> ETFSGGCLFDEPYSTCGYSQSEGDDFNWEQVNTLTKPTSDPWMPSGSFMLVNASGRPEGQRAHLLLPQLKENDTHCIDFHYFVSSKSNSPPGLLNVYVKVNNGPLGNPIWNISGDPTRTWNRAELAISTFWPNFYQVIFEVITSGHQGYLAIDEVKVLGHPCTRTPHFLRIQNVEVNAGQFATFQCSAIGRTVAGDRLWLQGIDVRDAPLKE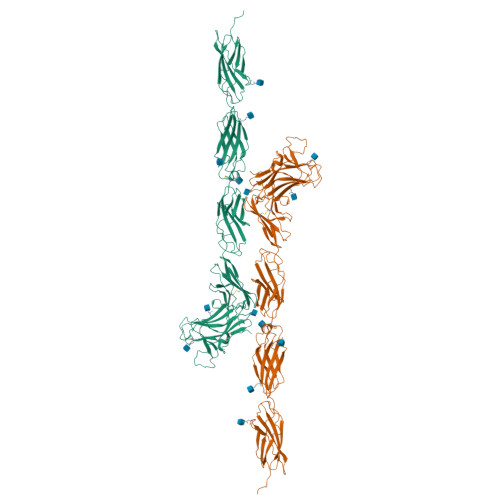IKVTSSRRFIASFNVVNTTKRDAGKYRCMIRTEGGVGISNYAELVVKEPPVPIAPPQLASVGATYLWIQLNANSINGDGPIVAREVEYCTASGSWNDRQPVDSTSYKIGHLDPDTEYEISVLLTRPGEGGTGSPGPALRTRTKCADPMRGPRKLEVVEVKSRQITIRWEPFGYNVTRCHSYNLTVHYCYQVGGQEQVREEVSWDTENSHPQHTITNLSPYTNVSVKLILMNPEGRKESQELIVQTDEDLPGAVPTESIQGSTFEEKIFLQWREPTQTYGVITLYEITYKAVSSFDPEIDLSNQSGRVSKLGNETHFLFFGLYPGTTYSFTIRASTAKGFGPPATNQFTTKISAPSMPAYELETPLNQTDNTVTVMLKPAHSRGAPVSVYQIVVEEERPRRTKKTTEILKCYPVPIHFQNASLLNSQYYFAAEFPADSLQAAQPFTIGDNKTYNGYWNTPLLPYKSYRIYFQAASRANGETKIDCVQVATKGAATPKPVPEPEKQTDHTVKGTKHHHHHH> MKRAVITGLGIVSSIGNNQQEVLASLREGRSGITFSQELKDSGMRSHVWGNVKLDTTGLIDRKVVRFMSDASIYAFLSMEQAIADAGLSPEAYQNNPRVGLIAGSGGGS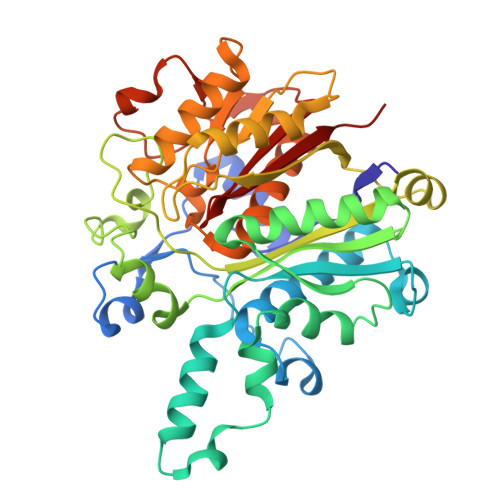PRFQVFGADAMRGPRGLKAVGPYVVTKAMASGVSACLATPFKIHGVNYSISSACATSAHCIGNAVEQIQLGKQDIVFAGGGEELCWEMACEFDAMGALSTKYNDTPEKASRTYDAHRDGFVIAGGGGMVVVEELEHALARGAHIYAEIVGYGATSDGADMVAPSGEGAVRCMKMAMHGVDTPIDYLNSHGTSTPVGDVKELAAIREVFGDKSPAISATKAMTGHSLGAAGVQEAIYSLLMLEHGFIAPSINIEELDEQAAGLNIVTETTDRELTTVMSNSFGFGGTNATLVMRKLKD>GGTGGTGGTGTGTTG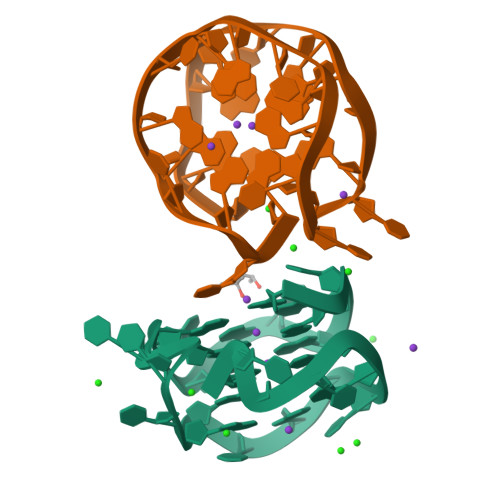GTGGTGGTGTG[2x]> QYSSNTQQGRTSIVHLFEWRWVDIALECERYLAPKGFGGVQVSPPNENVAIHNPFRPAWERYQPVSYKLCTRSGNEDEFRNMVTRCNNVGVRIYVDAVINHMCGNAVSAGTSSTCGSYFNPGSRDFPAVPYSGWDFNDGKCKTGSGDIENYNDATQVRDCRLSGLLDLALGKDYVRSKIAEYMNHLI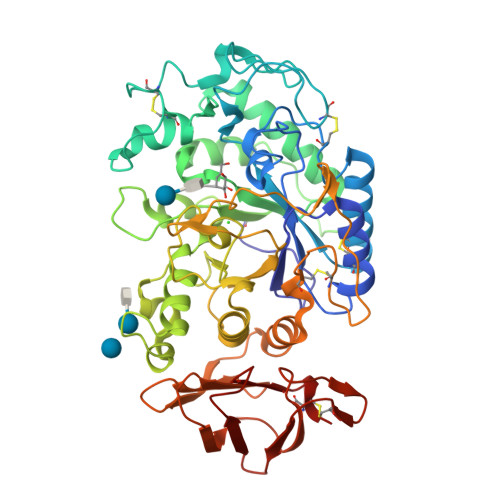DIGVAGFRIDASKHMWPGDIKAILDKLHNLNSNWFPEGSKPFIYQEVIDLGGEPIKSSDYFGNGRVTEFKYGAKLGTVIRKWNGEKMSYLKNWGEGWGFMPSDRALVFVDNHDNQRGHGAGGASILTFWDARLYKMAVGFMLAHPYGFTRVMSSYRWPRYFENGKDVNDWVGPPNDNGVTKEVTINPDTTCGNDWVCEHRWRQIRNMVNFRNVVDGQPFTNWYDNGSNQVAFGRGNRGFIVFNNDDWTFSLTLQTGLPAGTYCDVISGDKINGNCTGIKIYVSDDGKAHFSISNSAEDPFIAIHAESKL> LEHHHHHHMDTTQVTLIHKILAA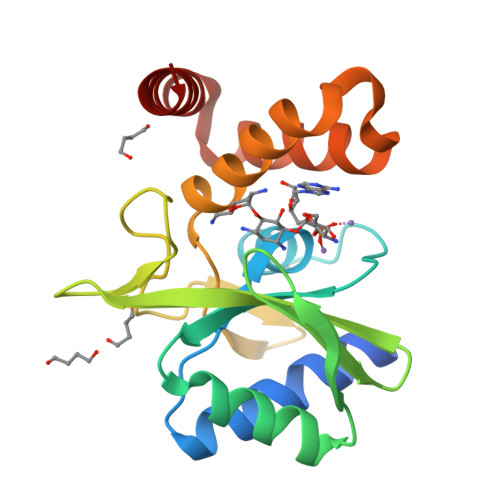ADERNLPLWIGGGWAIDARLGRVTRKHDDIDLTFPGERRGELEAIVEMLGGRVMEELDYGFLAEIGDELLDCEPAWWADEAYEIAEAPQGSCPEAAEGVIAGRPVRCNSWEAIIWDYFYYADEVPPVDWPTKHIESYRLACTSLGAEKVEVLRAAFRSRYAA> GSHMLKGQEFAPSHQQVYAPLRADGDKPRAHLTVVRQTPTQHFKNQFPALHWEHELGLAFTKNRMNYTNKFLLIPESGDYFIYSQVTFRGMTSESSEIRQAGRPNKPDSITVVITKVTDSYPEPTQLLMGTKSVSEVGSNWFQPIYLGAMFS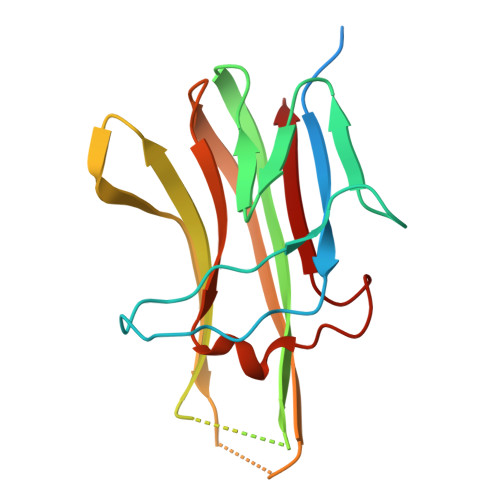LQEGDKLMVNVSDISLVDYTKEDKTFFGAFLL>MALLKRVVSEVVATFLLVFMTAGAAGISGSDLSRISQLGQSIAGGLIVVVMIYAVGHISGAHMNPAVTLAFAVFRHFPWIQVPFYWAAQFTGAIAASFVLKAVIHPVDVIGTTTPVGPHWHSLVVEVIVTFNMMFVTLAVATDTRAVGELAGLAVGSAVCITSIFAGAISGGSMNPARTLGPALASNRFDGLWIYFLGPVMGTLSGAWVYTFIRFEDTPREGSSQKLSSFKLRRLRSQQSIAADDVDEME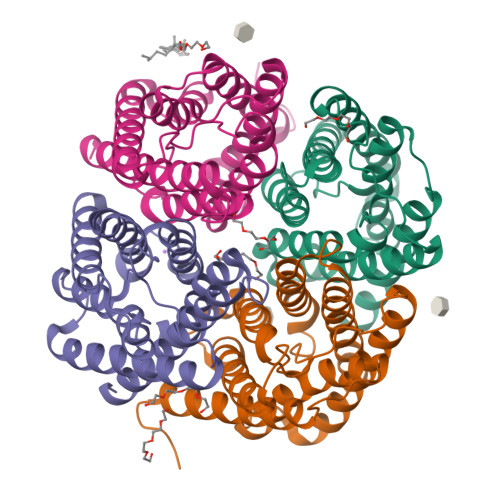NIQV[8x]>MGRENVLPVHNDVYEDFVFTTPYFQPESTFKSVPKLFSDILLGGVEWVYTTSESVLAYDYKLWYLWSGVSNLDESFDMFFNQYWALSLSTSVFQLFYAVILDRYLSVLFQNTPYTNDWFRMMLHSKETALIWLYHPELSWHINGLNQFFTYFYGGILEFVYFDKSNPDMCILVHTLWIHLLILFLIFTGFVTILFSFYGNPNTEENTIDSDYLAASGTVEAEKEITSIDDYLGLVFAIAYVFGVFFYVHGWTSMLSHAVLLLSCYSIIIMFLFILGMPTLLLYDFGIFFLAYLKGAGKYISSVAEMMFDYTACLVFYIRILAQWIRVVLMVVTFISLSHYVSDFDITNSALIGSENQSDSMNELNTNFSMTYYILTVLPGKFIYWIYEILHTFFVVCSQFVAFFAIVFWLFLFLYTFFIIEKHEDFFSKKREERKKKLKELWNLKN[2x];>[2x]MHSTLRVFTKNNCLSFTNMNRFSTAAQVAQANYSKFRADYSASVAAFQQRIKTIEKENTGSMKKPMAKAYEHPYNSEHHPLNFSAVKIAETFHDFIGPEQVSPHYESFAMSRKFLLTFWGGFFVLNFGMATVDLNWIMKSTYIPWIFWFQLMYFYVEGKNSMFMPLLQRFYRRAAANEIFTMEAFYHENIENKLRNLMRITKGQLEYWDIHTSYGEIRADSINNFLANEYLRLQSHITSRALNILKQAQAYETMNQAALLQKLIDDATSAIDNALKGDKKAEVLARSLDSAIDGLSKGYMDYQNDPLLPLILSSIEANVKKITTLSAQEQANLIGLTAEQLKSIKENDVRARKEFLESQPKLDNNLKNIESVKKILATWGK;>[2x]MITILDYLFLLDLNDDLTRKAVFEQVIIFIFIYCTMNFLAWSTVVELIWPTHFFNRRHSSSQEFIRFRTYTEVLLKISAYNDFFYVLNNYYYNQKLILKN;>MSMLAKIAKNVVKTQALKNTTAAQTPSFQAPGNQDKILKWISTLSNKATTGESRSYCTQLSSLVSFYNKQHVEQIPTIDFNEWKSVISTQGLVDKVKENYESLIKEQYNTDAISKQISSASSKALDDIENELSFHAAIWLNAYADYTMFLFELEEYNDPNDYLMHENFDFFRGLETELEELTETHNYIPGAKDDVNLRGYLATQFAWGKKVISFYRHPADDFKCAKATKNMLGR[2x];>[2x]MIHCLRNIRTVSALQSKISYNLGGGNKRKKTSGDLDNYDVLFVGANLGGICSNHFDKDTHGKYKCFVSFDQPINQIYSVRIPYEQQRVRKSEYIHFSKKSINQFTPSEMLAVKEILPEQNAVVLSSGRRIGYNQLVLATGLKHDFSQIKGFYEALEHPEHPVYANRDPETWRSAQHKYSKYISNFKSGDGYFCIPEYPYAGEVECFNFFVSDEVWKWAQHHGALSPKHTFTIVNANEKFVHYCDSADAFIKERLEKRGIRVEYNTKLLEVHQDGQKATFINTKTGEKSVRDYNNLYSIVPSKRQEFLDKAGLTNGNGLLNVDHQTLQHKKYKNIFGLGDAADLPTTKTFWAGWYQIAVVRNNVKRNLQGQTLNAHYDGFSKVPLFTGHQTLTYVAHSYGGVGNWQHLKHNNGGILAWMRYRSWAKGMAKKFQDFYNGARLGPPYHKVLKSFPELPGSPESQQSSGISKYFPTKTENKAAH;>[2x]MSLHEKMQTDYLWVKDHSQADSWAKARTHGYNYIAHTVPNKKERYEMIWRSMGKSTDWELEKFRLGKKFPDRGNKRRWFKNLFRLIKNPMGYIFWKTYKARLAKPSLIVTSMFIGFTLGFIKLKAQSIAYSKKQYATLRAGKNIEGSGQVHFGYHDQKWGMPAIPMFQLMYYELPGNSIVVNPCRNQNYRLYFEMRKKLGILPA;>[2x]MINRSTAFISKNLRQANLTQSSLAMKTQYNQMGFSSDNPYNKRWEYKWKHSYYTYPRDYEHTEVRKPQDSKDVPPIYFAYYKDFVDRWLPGMNMWWQRRHRIFDKFNVYFLPGMSLFFYQFADLALGFKIMAAFPLFLAYTRIRDKTLDPDFKETYLRDMIYQNPEITKYFNEETIHVLDYEFEYLPGYLCPEKFPEYQNKTWQFFNTDTAQAEGFFKFGDVESGATMTLKFKTMPIPGKFRYQVGEPFYFYDLRAEIKCDGVYKEVVLVDEKESLKKIRPFLFLI;>MQQRKKIYLRQKRKIYIQLKNKEKKKNNQFIQKREKMGYKIRNKSIFWTRAGWKNNWHPKNFNAPRPSYGEFTMGIRCRNDHHSFLRYVQTYRNMSRHCKQYFLGDKQLEETFILGLRSLFLVPYDSQCLTDQIKHGGERRFVDQLDRDFELISYNTHPYQLFTYTVRNEHLAWKNEQYEKIQKGEKTFEQELLDYLDEQVLAEKAKLRDGQNFSIERMTEIALHVFRKARAGKVRPAQDVRGPDGNVNDFLEQRRPFEHPNPTGVTH[2x];>[2x]MNPIQKAWLKILEPVSYVINEKMAKRTGIIGKLGRFFAIGPREYGVHPINRMFIFMNRKYMAFQAVALHRYSFVKSLTHNGFHMLRVFRHFAFVLPATVLAGLGLFVYWGDDNKCYSPDRFPYLKKRAGDMALPLNSLNQRTSAHYIEINAIYGAEMMKRYHKVWENIIEERSKATDQEKKTRYAHPSYQYSPLPVVSIPNVLNPLNLQ;>[2x]MSENKAPGQIYAYDIHNTHYPYVNIKQDSQTQLLASFRRSIASINPFSYRQVPSQDRAAFGLRWGNAWYAPNPYPNGIHFDRVFPTHYDPLAETNRTKANLQLIKYAPGNYSTLVVTSEKLPRPCIRTIQNYRRCQMVNGTEKCNSEAQDILAICPNWALDHMKEKVRFYTKALAINNQTYIRAMQVEEYNQGRTVADVAPKTWIHGTRQHLRPDTMWADDRYTNITQTEINEAIKRVEARKAREHEKKPVEQANVNANTGEQPVRVEKSLYP;>[2x]MWYKYFSKQSWNLRVWRKANLKYNQDDFGMTQPKYIARFGDFRFRLVRTEGALRGCMFFVGFGCFSIINYLYGRYGYIINESSQKRAAQDLLDNDMAADKILFKNRVGAPTRPLRSLDDMMAFLSGSATYDQLADYASYNHAMDVNQDQQAGLDSWMSEKDKNMVKYYQRSLGKKVEGI;>MPVKEGQAKLWFSTKEEADAYDDKMISNIELKSQDYEDENFSPVFNRKTQEYFLEPSEKFKSDFAELLRPLRSLSFNQVVDRYVLIPPNHTFYRNWTYEKFLGGFGLSYLILRELPLRNFYARVFVMYAFAAKVLDHLGNPFPFSGHGQIVAAADRWNHWDVRCYDNVMKALKYIRIPTVQNNIPEATRWYGRQPGHLLRADTYWIPNLVSQRFAKHQPAHWDGTQNMPIFRLADPKHKDSYMVQFR[2x];>MDNYFTAITLLGLRDQNLPPFKDARLQRYKSIKKMIDLIETTTKLAPPMPVELFMLNPTDPEWDDDMTYPTITHATALYKSSALAGNLFLYAYNYNNFTANIRLRTMRYLFPVVSLAIFGNIYWDYRSQLVKVNLFDEYIQARAQELVKQNEYLLEHEDVKRYVWWYEDLKETLARVHRQANNHKACDFKDSEIILQDFIRRYTNPKDNLPIKFHPQGQTF[2x];>[2x]MEGFIQNKRKKEKEGEEEEESKEKRKQINQLNKQKQEEEKIYQQKKDQKRKKYLYQRKEMTIFAETWEASEYQYRNKANLKTLPVNHLGKLAELKFDFVEYKAHQLIACHLYERMTIHCMNQYGLFKDFYRPECLDAQYYFKTCVELNAAYGIQKKFFPEHFVGSPYARPVPQFQQLGL;>[2x]MKQKINKLLKNKGVQDKYKYLSKLILLDQEIKGKIKRKNKKEKQKRKNKLILEEMQNTTNIVHVPVHMGHTHYFDYIDSFPKLKEGPTLEENHITNQKILREQLISGQQGLEQNLCLRNCFKLSQKRYIEFCLDRKCGGADFQRAATILGYTKN;>MSNIFLELQDGDKTVYTHTSLIEESKQEQIQAIYDKVPQWTNGGRFLGFWLSMEAVNRVQSVAKLPIYYRAGIVATSTLLGGLVSSLVFWKSGNENQVAKLANGAPVYLKKWEVPELSKLYFFLDDDNNFKPSLNHHAVTQGRQYYKIYQHN[2x];>[2x]MFRNILSLVTKPSKLSQKTFYNFAAAKNEVQVSKKQQQAGAKRDLTQYVEGQIVNRNQLTLKKQEDIEQYVLKLVRGYFRTTNKQGLNINSVLQDHGLDEFDSIELAMQVEEDLGYVISAETIPVLNKVKHFVNYINHVEQFKAENGKAPIA;>MSQDPKIVNPQLWPNPNKLRFADLYKYQGVEMKKINDSIKNYKAAKFYIGGILGGCLVFKFFIDAAVDKYIFGENGNGGKFLEMQTINSNYDYYYNRQFQRMRYLTEDPAGDDPLQKTKDEHLVDLGFIPKVFGANVEVRKRAPHDKYL[2x];>[2x]MNSLSSKKANSLVFKSIRNFTLQWGSLAERPMVDRVMSTSTWPVPYYQRLFKAYPIREKKDKMSLLLSDIDIDDTNWYQAKDFLRGSFRGRQIVDYVENNIASNTYILIQQDVANMAKAYVHDICGYIDVANKENVRILSKGDLI;>[2x]MNRSVNIAKNLIQTYRAMSVQSRFAFSTREEEWLDKRTKSQEKVYFDQEDRKAMKRLLEKLNTTSKFVEDSEYLAPQNLEVENILKRYHINYTQALIDELVDWKTGKN;> MKMEYLQSEEKKDAINKQIHKKEEKEEKEIKIKRKNKVKQRIQIINQIKKYIEAKQQKKQIQSKNQRKYKGRMINTRKQVFKCLWGAQPAYNFSRIINHLRGDPVYQDNTKDVSLRGTFLRGKYDDLPTMIFFTEACDLTANWIPFFTNPQYDILAHRNVWLLNPRNFGNSDRHPSFDLQEMSDDVMRFMYSQKISMATLGGHGIGGKIALAVGCYHAERVTGVFSIDSSPMDQRYHEAFKEFKGYVNALTEINFKTWSDKDVKVFLKENIKDPKWRSIFTNNISKNAKTQSDSFNFEINYLNHNLNFNKADSLGNWAVKNGIYTGRAHFIFPEYSRWVHLATNTLPMHKVCARVKGFGHDIFYVQGDENPLNHWVYDFENYANVVASKLNKFLHSYDGVHALLKDRTEIGNFMIPDRIKSRNDSKHIYGDYSPAHLHHNWRFNHIYEKHDELDKKLNEQ

The F-type ATP synthase (F1Fo-ATP synthase) is responsible for generating most of the cellular adenosine triphosphate (ATP) from adenosine diphosphate (ADP) and inorganic phosphate through rotary catalysis. In eukaryotes, ATP synthases are found in the inner mitochondrial membrane. The type III ATP synthase was detected in ciliates where it induces tubulation of the cristae membranes. In this study, we present the cryo-EM structures of the type III ATP synthase dimer and tetramer with associated lipids from the model organism Tetrahymena thermophila in complex with the natural inhibitor IF1.

Using masked refinements, the resolution of different regions reached 2.5–3.1 Å, allowing de novo modelling. In the Fo-subcomplex, 6 out of 7 conserved subunits are extended and 13 subunits have no structural equivalents in other types of ATP synthases. Our structure of the dimer reveals that, unlike in all the previously investigated complexes, the monomers of the membrane-embedded Fo-subcomplex are not identical to each other. The commonly observed C2-symmetry is broken by the accommodation of a single ATPTT2 subunit at the dimer interface that anchors the IF1. Markedly standing out is ATPTT2, observed only as a single copy in the dimer. ATPTT2 contains a sequence-conserved core, adopting a classical α/β hydrolase fold, although with an inactive catalytic triad. At the C-terminus, two helices of each IF1 copy form a four-helix bundle, mediated by ATPTT2. Apart from the protein subunits, we also assigned in the Fo-subcomplex 30 cardiolipins, 6 phosphatidylcholines, 4 phosphatidylethanolamines, and 2 coenzyme Q (CoQ) molecules. Six of the cardiolipins are deeply embedded within the Fo-subcomplex, sequestered from the bulk membrane and instead acting as structural components of the ATP synthase dimer structure. Unexpectedly, we discovered a Mg-ATP molecule bound as a structural Fo-component on the matrix side, serving as a hub of interactions connecting subunits a, k, ATPTT3 and ATPTT4.>QQFLSQFYLNDQDVYLTSNVGGPIQDENSLSAGQRGATLLQDFIFREKIQRFDHERVPERAVHARGTGAHGTFTSYGDWSNLTAASFLSAEGKETPMFTRFSTVAGSRGSADTARDVHGFATRFYTDEGNFDIVGNNIPVFFIQDAILFPDLIHAVKPRGDNQIPQAATAHDSAWDFFSQQPSVLHTLLWAMAGHGIPRSFRHVNGFGVHTFRLVTDDGKTKLVKFHWKGLQGKASFVWEEAQQTAGKNADFMRQDLFQSIQAGRFPEWELGVQIMQEQDQLKFGFDLLDPTKIVPEELVPVTILGKMQLNRNPMNYFAETEQVMFQPGHIVRGVDFTEDPLLQGRLFSYLDTQLNRHGGPNFEQLPINRPRAPIHNNNRDGAGQMFIPLDPNAYSPNTENKGSPKQANETVGKGFFTAPERTASGKLQRTLSTTFENNWSQPRLFWNSLVNAQKEFIVDAMRFETSNVSSSVVRDDVIIQLNRISDNLATRVASAIGVEAPKPNSSFYHDNTTAHIGAFGEKLAKLDGLKVGLLASVNKPASIAQGAKLQVALSSVGVDVVVVAERMANNVDETYSASDAVQFDAVVVADGAEGLFGADSFTVEPSAGSGASTLYPAGRPLNILLDAFRFGKTVGALGSGSDALESGQISSERQGVYTGKNAGDAFAKDIKSGLS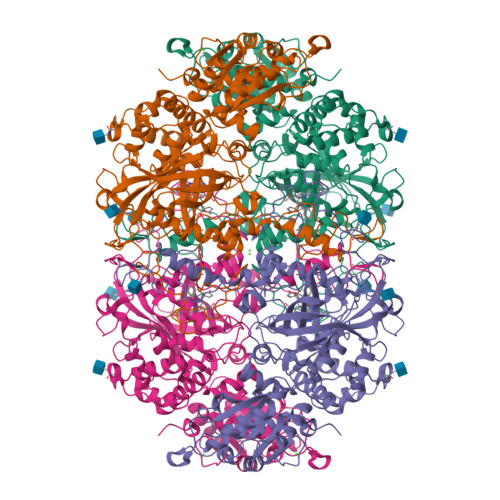TFKFLDRFAVDE[2x]>MITTKTVNGVQIAFDDQGHEPGPVFVTLSGWAHDLRAYDGMLPYLRAAQRTVRVCWRGHGPDRNLVGDFGIDEMAADTIGLLDALEVDSFVPIAHSHGGWAALEIADRLGAQRVPAVMILDLIMTPAPREFVAALHGIQDPERWKEGRDGLVQSWLAGTTNQAVLDHV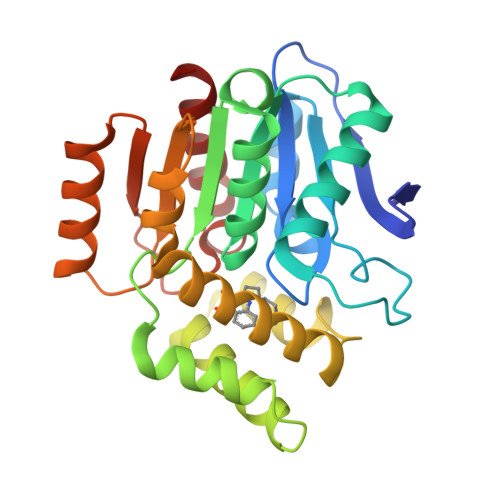RYDSGGHGFDMWARAGRVIDEAYRTWGSPMRRMEALAEPCAIRHVFSHPKIGEYDALHDDFAARHPWFSYRRLGGETAFPGIELPQQVAAEAIDLLAGARI[3x]BERENIL 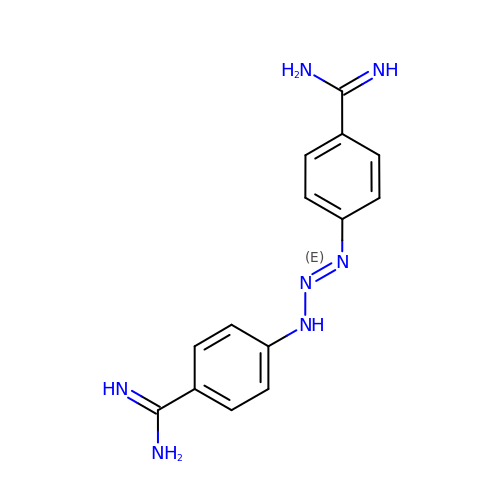| C14 H15 N7 | XNYZHCFCZNMTFY-UHFFFAOYSA-N> YQGGGEEM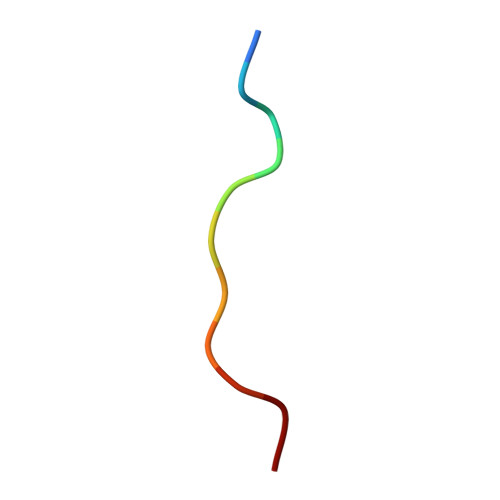ALP>GSHMSQKFDVVVIGAGPGGYVAAIRAAQLGLKTACIEKYIGKEGKVALGGTCLNVGCIPSKALLDSSYKYHEAKEAFKVHGIEAKGVTIDVPAMVARKANIVKNLTGGIATLFKANGVTSFEGHGKLLANKQVEVTGLDGKTQVLEAENVIIASGSRPVEIPPAPLTDDIIVDSTGALEFQAVPKKLGVIGAGVIGLELGSVWARLGAEVTVLEALDKFLPAADEQIAKEALKVLTKQGLNIRLGARVTASEVKKKQVTVTFTDANGEQKETFDKLIVAVGRRPVTTDLLAADSGVTLDERGFIYVDDHCKTSVPGVFAIGDV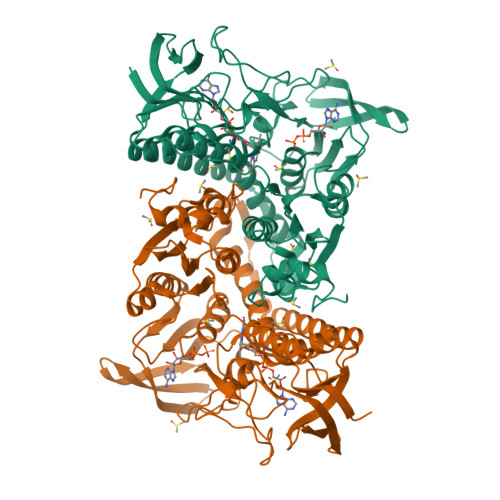VRGAMLAHKASEEGVMVAERIAGHKAQMNYDLIPSVIYTHPEIAWVGKTEQTLKAEGVEVNVGTFPFAASGRAMAANDTTGLVKVIADAKTDRVLGVHVIGPSAAELVQQGAIGMEFGTSAEDLGMMVFSHPTLSEALHEAALAVNGHAIHIANRKKR[4x]> NVLPSELPAGVDWRSRGCVTPVKDQRDCGSCWAFSTTGALEGAHCAKTGKLVSLSEQELMDCSRAEGNQSCSGGEMNDAFQYVLDSGGICSEDAYPYLARDEECRAQSCEKVVKILGFKDVPRRSEAAMKAALAKSPVSIAIEADQMPFQFYHEGVFDASCGTDLDHGVLLVGYG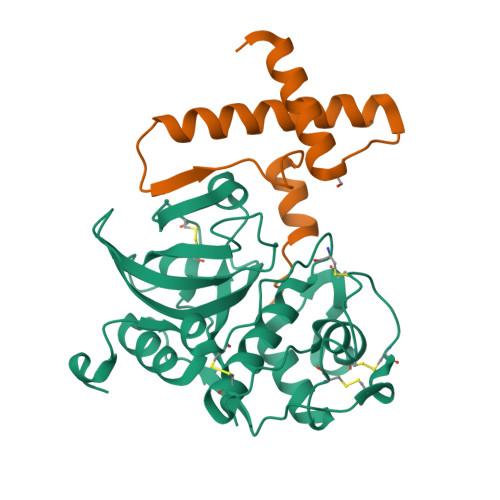TDKESKKDFWIMKNSWGTGWGRDGYMYMAMHKGEEGQCGLLLDASFPVM;> MRGSHHHHHHGSIWEWKEAHFQDAFSSFQAMYAKSYATEEEKQRRYAIFKNNLVYIHTHNQQGYSYSLKMNHFGDLSRDEFRRKYLGFKKSRNLKSHHLGVATELL> MASVHGTTYELLRRQGIDTVFGNPGSNALPFLKDFPEDFRYILALQEACVVGIADGYAQASRKPAFINLHSAAGTGNAMGALSNAWNSHSPLIVTAGQQTRAMIGVEALLTNVDAANLPRPLVKWSYEPASAAEVPHAMSRAIHMASMAPQGPVYLSVPYDDWDKDADPQSHHLFDRHVSSSVRLNDQDLDILVKALNSASNPAIVLGPDVDAANANADCVMLAERLKAPVWVAPSAPRCPFPTRHPCFRGLMPAGIAAISQLLEGHDVVLVIGAPVFRYHQYDPGQYLKPGTRLISVTCDPLEAARAPMGDAIVADIGAMASALANLVEESSRQLPTAAPEPAKVDQDAGRLHPETVFDTLNDMAPENAIYLNESTSTTAQMWQRLNMRNPGSYYFCAAGGLGFALPAAIGVQLAEPERQVIAVIGDGSA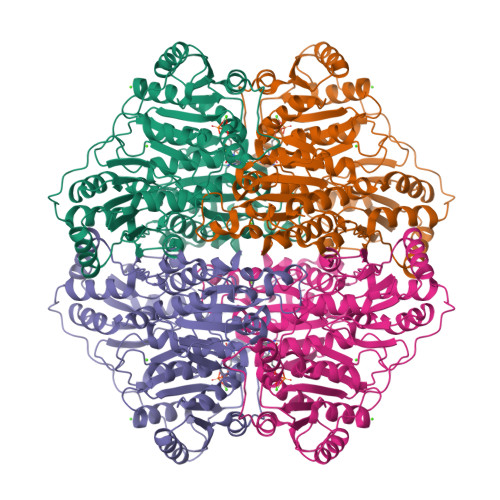NYSISALWTAAQYNIPTIFVIMNNGTYGALRWFAGVLEAENVPGLDVPGIDFRALAKGYGVQALKADNLEQLKGSLQEALSAKGPVLIEVSTVSPVK1-methyl-5-(phenylamino)-1,2-dihydro-3H-pyrazol-3-one 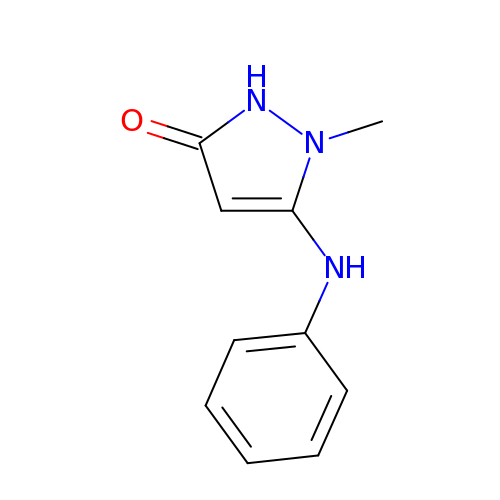| C10 H11 N3 O | JAPKWXYUAJYHCE-UHFFFAOYSA-N N-[4-(3-chloranyl-4-cyano-phenoxy)cyclohexyl]-1,1,1-tris(fluoranyl)methanesulfonamide | C14 H14 Cl F3 N2 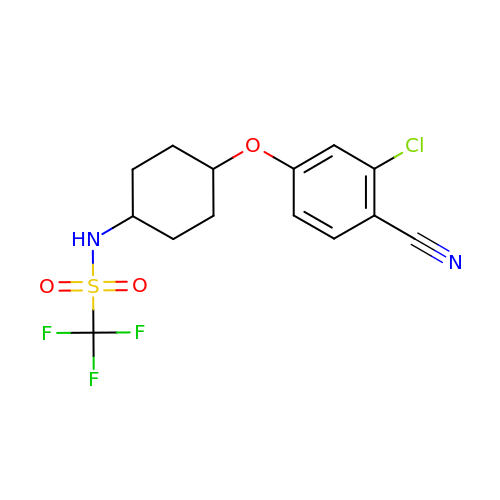O3 S | AMFHXCAGSKYZAM-XYPYZODXSA-N>GAKRPRTTITAKQLETLKNAYKNSPKPARHVREQLS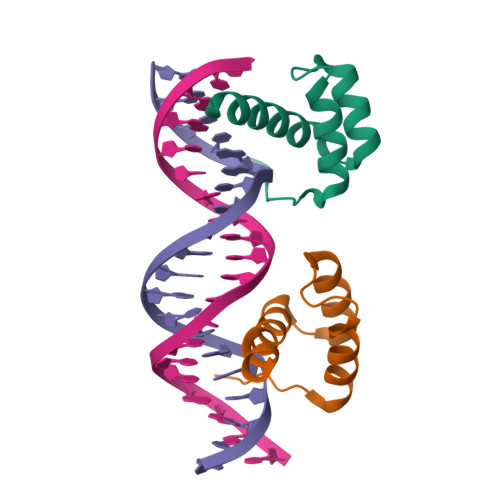SETGLDMRVVQVWFQNRRAKEKRLK[2x]Split inteins catalyze protein trans-splicing by ligating their extein sequences while undergoing self-excision, enabling diverse protein modification applications. The Aes123 PolB1 intein, a representative of the rare cysteine-less split inteins, is of particular interest due to its resistance to oxidative conditions and orthogonality to thiol chemistries. The cysteine-less Aes123 PolB1 intein (in short: Aes intein) found inserted in PolB-type DNA polymerase genes from T4-like bacteriophages of Aeromonas salmonicida shows only about 30% splicing efficiency relative to its PN12. In this work, we identify β-sheet-dominated aggregation of its N-terminal intein fragment as the origin of its low (~30%) splicing efficiency.

To this end, we also solved the crystal structure of an AesN-AesC fusion at 1.38 Å resolution to confirm that selected residues indeed formed β-sheet structures and to choose sterically fitting substitutions. Interestingly, two of the three strongest APRs within AesN (APR1 & APR3) are directly in contact with AesC. The structure also confirmed the presence of the recently discovered motif NX histidine as a unique residue conserved in cysteine-less inteins. We then designed mutations within the predicted regions of the C-terminal half of AesN. Amino acids were changed to ones with a lower propensity for forming β-sheets. Mutations towards polar and in particular positively charged side chains were preferred to avoid counteracting the electrostatically driven association with the AesC precursor. In the following, we focused on the mutant 1P(T69K/F75H/M118N), from now on termed CLm intein (cysteine-less monomeric; 15P), as it retained the best ultra-fast splicing activity with t½ = 16.3 s, only about 3.3-fold slower than the WT, and reached 89% splicing efficiency.

>IDTDAVVGDTIIDVSGKKMTIAEFYDSTPDVFMRRNDEARDWVKRVGGKTSLSVNTYSGEVERKNINYIMKHTVKKRMFKIKAGGKEVIVTADHSVMVKRDGKIIDVKPTEMKQTDRVVKWMLTGSHMIEFIEFEIEDLGVMEIDVYDIEVDGNHNFFGNDILVHASVYLNKL[2x]(2R,3R)-2,3-bis{[(2E)-3-(3,4-dihydroxyphenyl)prop-2-enoyl]oxy}butanedioic acid | C22 H18 O12 | 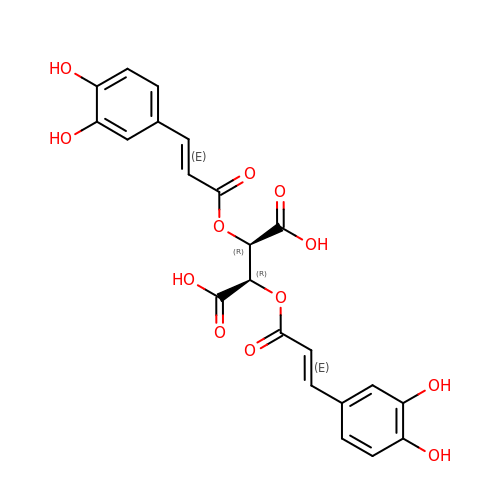YDDGKXBLOXEEMN-IABMMNSOSA-N>MGSSHHHHHHSSENLYFQGHMADQDHAQLLHVLGIENLRRGADGNTDSPFAANTDEAKANTALD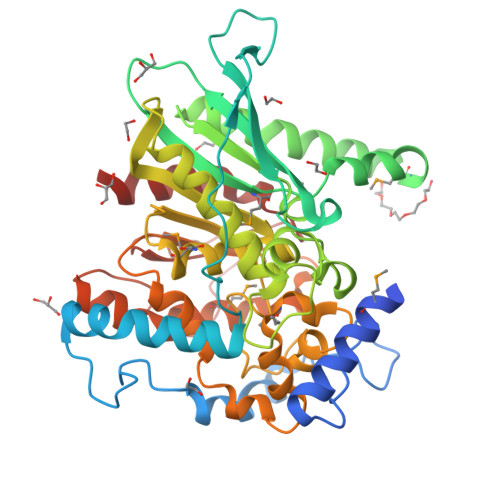SLPPLLTSVSGQAIASATDWEANRPALLNTFSQEIYGYVPGGAPELHWKAGSTTPIDDSGTSAIRQHFTSTLVHPENAALNLSLNFTLVLPKSNKPVPVVVVMSFDPGIWERFRDRMPAERYAQIQADNARWREQVVNAGWGYAEIIPTEFQADSGDGLSQGIIGFVNNGKPRNPTDWGALRAWAWSASQVLTYLQTDSRVAADRISVHGHSRFGKAALVAMAFDNRFAAGFISSSGEGGAKLWRRNFGEQVGNLAGAGEYHWMAGNFVKYAGPKKVNDIPVDAHQLLALCAPRPVLVSVGSQGESWVDPKGMLLAAYHATPAYALFGEQGVTQNELPAVGNGLLAGKLAFRQHEGGHTPAPNWETFITFATRQWA[3x]Bacterial multiheme cytochromes (MHCs) attract much attention for their contributions to extracellular electron transfer whereby electrons are exchanged across the cell boundary and consequently between internal enzymes and external redox partners. These processes evolved to allow the capture of electrons for anabolic reactions and the release of electrons from internal oxidation during anaerobic respiration. Thus, we investigated whether amber suppression in MR-1 could produce ncAA-containing MHCs and, specifically, variants of the MtrC protein, which contains ten c-type hemes. MtrC is found on the outer surface of MR-1 cells. MR-1 cells typically present MtrC tightly bound to the external face of the outer membrane spanning the MtrAB porin-cytochrome complex.

The structure of wtMtrC was inspected to identify surface residues that might be changed to ncAAs with limited effect on the MtrC structure. Residue A293 in Domain II and E344 and A430 in Domain III were chosen, Figure 2C. Thus, site-specific replacement of MtrC surface residues with BocK has no discernible impact on the protein structure. By contrast, there was no detectable FMN reduction for ΔmtrC/omcA MR-1 cells cultured in the absence of wtMtrC. Cells from cultures augmented by MtrC344BocK and MtrC430BocK also displayed FMN reduction rates comparable to those of MR-1, Figure 5C. Thus, our results indicate that MtrC344BocK and MtrC430BocK retain the structure and redox activity of wtMtrC. A crystal structure of the homologous MtrCAB complex purified from Shewanella baltica OS18542 shows that MtrC Domain III, which contains residues 344 and 430, makes no contribution to the binding with MtrAB. This is consistent with the ability of wtMtrC, MtrC344BocK, and MtrC430BocK to restore FMN reduction activity to ΔmtrC/omcA MR-1 cells by associating with MtrAB in the outer membrane.

> MKFKLNLITLALLANTGLAVAADGGSDGNNGNDGSDGGEPAGSIQTLNLDITKVSYENGAPMVTVFATNEADMPVIGLANLEIKKALQLIPEGATGPGNSANWQGLGSSKSYVDNKNGSYTFKFDAFDSNKVFNAQLTQRFNVVSAAGKLADGTTVPVAEMVEDFDGQGNAPQYTKNIVSHEVCASCHVEGEKIYHQATEVETCISCHTQEFADGRGKPHVAFSHLIHNVHNANKAWGKDNKIPTVAQNIVQDNCQVCHVESDMLTEAKNWSRIPTMEVCSSCHVDIDFAAGKGHSQQLDNSNCIACHNSDWTAELHTAKTTATKNLINQYGIETTSTINTKTKAATISVQVVDANGTAVDLKTILPKVQRLEIITNVGPNNATLGYSGKDSIFAIKNGALDPKATINDAGKLVYTTTKDLKLGQNGADSDTAFSFVGWSMCSSEGKFVDCADPAFDGVDVTKYTGMKADLAFATLSGKAPSTRHVDSVNMTACANCHTAEFEIHKGKQHAGFVMTEQLSHTQDANGKAIVGLDACVTCHTPDGTYSFANRGALELKLHKKHVEDAYGLIGGNCASCHSDFNLESFKKKGALNTAAAADKTGLYSTPITATCTTCHTVGSQYMVHTKETLESFGAVVDGTKDDATSAAQSETCFYCHTPTVADHTKVKMSAWSHPQFEK>GSKKHTGYVGLKNQGATCYMNSLLQTLFFTNQLRKAVYMMPTEGDDSSKSVPLALQRVFYELQHSDKPVGTKKLTKSFGWETLDSFMQHDVQELCRVLLDNVENKMKGTCVEGTIPKLFRGKMVSYIQCKEVDYRSDRREDYYDIQLSIKGKKNIFESFVDYVAVEQLDGDNKYDAGEHGLQEAEKGVKFLTLPPVLHLQLMRAMYDPQTDQNIKINDRFEFPEQLPLDEFLQKTDPKDPANYILHAVLVHSGDN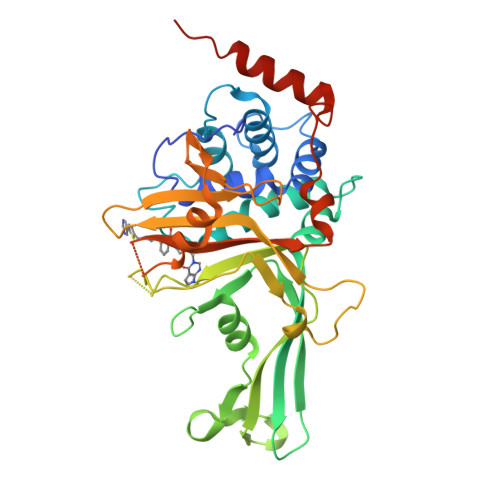HGGHYVVYLNPKGDGKWCKFDDDVVSRCTKEEAIEHNYGGHDDDLSVRHCTNAYMLVYIRESKLSEVLQAVTDHDIPQQLVERLQEEKRIEAQKRKERQE[2x]1-[4-chloranyl-3-(trifluoromethyl)phenyl]-3-(5-oxidanylidene-6-pyridin-4-yl-pyrido[2,3-b][1,5]benzoxazepin-9-yl)urea | C25 H15 Cl F3 N5 O3 | 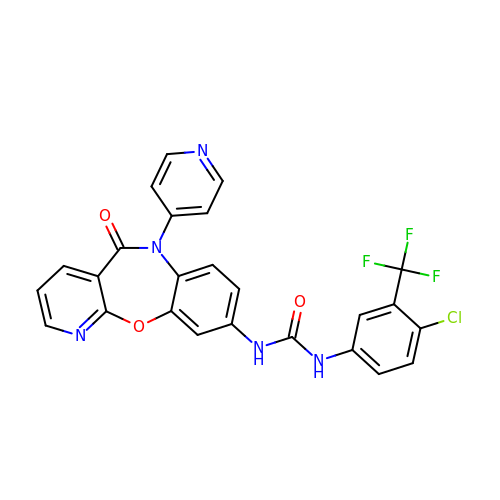NQHGDUGVQSAKOR-UHFFFAOYSA-N>[2x]YFQSMEAEDFECSSHCSELSWRQNEQRRQGLFCDITLCFGGAGGREFRAHRSVLAAATEYFTPLLSGQFSESRSGRVEMRKWSSEPGPEPDTVEAVIEYMYTGRIRVSTGSVHEVLELADRFLLIRLKEFCGEFLKKKLH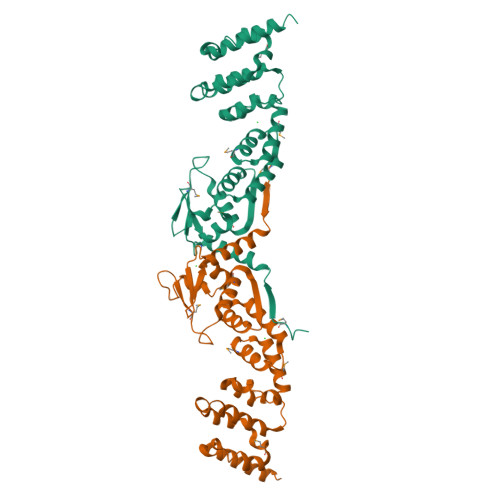LSNCVAIHSLAHMYTLSQLALKAADMIRRNFHKVIQDEEFYTLPFHLIRDWLSDLEITVDSEEVLFETVLKWVQRNAEERERYFEELFKLLRLSQMKPTYLTRHVKPERLVANNEVCVKLVADAVERHALRAENIQSGT> MDSLSVNQILYPEVHLDSPIVTNKIVAILEYARVPHAYSLEDPTLCQNIKHRLKNGFSNQMIINNVEVGNVIKSKLRSYPAHSHIPYPNCNQDLFNIEDKESTRKIRELLKKGNSLYSKVSDKVFQCLRDTNSRLGLGSELREDIKEKVINLGVYMHSSQWFEPFLFWFTVKTEMRSVIKSQTHTCHRRRHTPVFFTGSSVELLISRDLVAIISKESQHVYYLTFELVLMYCDVIEGRLMTETAMTIDARYTELLGRVRYMWKLIDGFFPALGNPTYQIVAMLEPLSLAYLQLRDITVELRGAFLNHCFTEIHDVLDQNGFSDEGTYHELIEALDYIFITDDIHLTGEIFSFFRSFGHPRLEAVTAAENVRKYMNQPKVIVYETLMKGHAIFCGIIINGYRDRHGGSWPPLTLPLHAADTIRNAQASGDGLTHEQCVDNWKSFAGVKFGCFMPLSLDSDLTMYLKDKALAALQREWDSVYPKEFLRYDPPKGTGSRRLVDVFLNDSSFDPYDVIMYVVSGAYLHDPEFNLSYSLKEKEIKETGRLFAKMTYKMRACQVIAENLISNGIGKYFKDNGMAKDEHDLTKALHTLAVSGVPKDLKESHRGGPVLKTYSRSPVHTSTRNVRAAKGFIGFPQVIRQDQDTDHPENMEAYETVSAFITTDLKKYCLNWRYETISLFAQRLNEIYGLPSFFQWLHKRLETSVLYVSDPHCPPDLDAHIPLYKVPNDQIFIKYPMGGIEGYCQKLWTISTIPYLYLAAYESGVRIASLVQGDNQTIAVTKRVPSTWPYNLKKREAARVTRDYFVILRQRLHDIGHHLKANETIVSSHFFVYSKGIYYDGLLVSQSLKSIARCVFWSETIVDETRAACSNIATT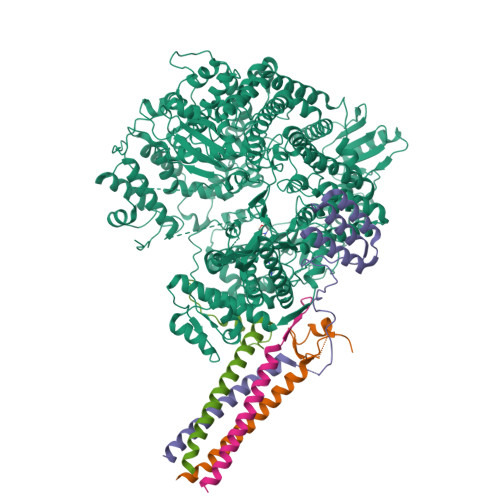MAKSIERGYDRYLAYSLNVLKVIQQILISLGFTINSTMTRDVVIPLLTNNDLLIRMALLPAPIGGMNYLNMSRLFVRNIGDPVTSSIADLKRMILASLMPEETLHQVMTQQPGDSSFLDWASDPYSANLVCVQSITRLLKNITARFVLIHSPNPMLKGLFHDDSKEEDEGLAAFLMDRHIIVPRAAHEILDHSVTGARESIAGMLDTTKGLIRASMRKGGLTSRVITRLSNYDYEQFRAGMVLLTGRKRNVLIDKESCSVQLARALRSHMWARLARGRPIYGLEVPDVLESMRGHLIRRHETCVICECGSVNYGWFFVPSGCQLDDIDKETSSLRVPYIGSTTDERTDMKLAFVRAPSRSLRSAVRIATVYSWAYGDDDSSWNEAWLLARQRANVSLEELRVITPISTSTNLAHRLRDRSTQVKYSGTSLVRVARYTTISNDNLSFVISDKKVDTNFIYQQGMLLGLGVLETLFRLEKDTGSSNTVLHLHVETDCCVIPMIDHPRIPSSRKLELRAELCTNPLIYDNAPLIDRDATRLYTQSHRRHLVEFVTWSTPQLYHILAKSTALSMIDLVTKFEKDHMNEISALIGDDDINSFITEFLLIEPRLFTIYLGQCAAINWAFDVHYHRPSGKYQMGELLSSFLSRMSKGVFKVLVNALSHPKIYKKFWHCGIIEPIHGPSLDAQNLHTTVCNMVYTCYMTYLDLLLNEELEEFTFLLCESDEDVVPDRFDNIQAKHLCVLADLYCQPGTCPPIQGLRPVEKCAVLTDHIKAEAMLSPAGSSWNINPIIVDHYSCSLTYLRRGSIKQIRLRVDPGFIFDALAEVNVSQPKIGSNNISNMSIKAFRPPHDDVAKLLKDINTSKHNLPISGGNLANYEIHAFRRIGLNSSACYKAVEISTLIRRCLEPGEDGLFLGEGSGSMLITYKEILKLSKCFYNSGVSANSRSGQRELAPYPSEVGLVEHRMGVGNIVKVLFNGRPEVTWVGSVDCFNFIVSNIPTSSVGFIHSDIETLPDKDTIEKLEELAAILSMALLLGKIGSILVIKLMPFSGDFVQGFISYVGSHYREVNLVYPRYSNFISTESYLVMTDLKANRLMNPEKIKQQIIESSVRTSPGLIGHILSIKQLSCIQAIVGDAVSRGDINPTLKKLTPIEQVLINCGLAINGPKLCKELIHHDVASGQDGLLNSILILYRELARFKDNQRSQQGMFHAYPVLVSSRQRELISRITRKFWGHILLYSGNRKLINKFIQNLKSGYLILDLHQNIFVKNLSKSEKQIIMTGGLKREWVFKVTVKETKEWYKLVGYSALIKD;>MAEEQARHVKNGLECIRALKAEPIGSLAIEEAMAAWSEISDNPGQERATCREEKAGSSGLSKPCLSAIGSTEGGAPRIRGQGPGESDDDAETLGIPPRNLQASSTGLQCHYVYDHSGEAVKGIQDADSIMVQSGLDGDSTLSGGDNESENSDVDIGEPDTEGYAITDRGSAPISMGFRASDVETAEGGEIHELLRLQSRGNNFPKLGKTLNVPPPPDPGRASTSGTPIKKGTDARLASFGTEIASSLTGGATQCARKSPSEPSGPGAPAGNVPECVSNAALIQEWTPESGTTISPRSQNNEEGGDHYDDELFSDVQDIKTALAKIHEDNQKIISKLESLLLLKGEVESIKKQINRQNISISTLEGHLSSIMIAIPGLGKDPNDPTADVEINPDLKPIIGRDSGRALAEVLKKPVASRQLQGMTNGRTSSRGQLLKEFQLKPIGKKMSSAVGFVPDTGPASRSVIRSIIKSSRLEEDRKRYLMTLLDDIKGANDLAKFHQMLMKIIMKSG[4x]>[8x]MTSVTSKQSTILGSDEIDLGRVIGELIDHRKLIISITSVFTLFAILYALLATPIYETDALIQIEQKQGNAILSSLSQVLPDGQPQSAPETALLQSRMILGKTIDDLNLQIQIEQKYFPVIGRGLARLMGEKPGNIDITRLYLPDSDDISNNTPSIILTVKDKENYSINSDGIQLNGVVGTLLNEKGISLLVNEIDAKPGDQFVITQLPRLKAISDLLKSFSVADLGKDTGMLTLTLTGDNPKRISHILDSISQNYLAQNIARQAAQDAKSLEFLNQQLPKVRAELDSAEDKLNAYRKQKDSVDLNMEAKSVLDQIVNVDNQLNELTFREAEVSQLYTKEHPTYKALMEKRQTLQEEKSKLNKRVSSMPSTQQEVLRLSRDVESGRAVYLQLLNRQQELNIAKSSAIGNVRIIDNAVTDPNPVRPKKTIIIVIGVVLGLIVSVVLVLFQVFLRRGIESPEQLEEIGINVYASIPISEWLTKNARQSGKVRKNQSDTLLAVGNPADLAVEAIRGLRTSLHFAMMEAKNNVLMISGASPSAGMTFISSNLAATIAITGKKVLFIDADLRKGYAHKMFGHKNDKGLSEFLSGQAAAEMIIDKVEGGGFDYIGRGQIPPNPAELLMHPRFEQLLNWASQNYDLIIIDTPPILAVTDAAIIGRYAGTCLLVARFEKNTVKEIDVSMKRFEQSGVVVKGCILNGVVKKASSYYRYGHNHYGYSYYDKKHHHHHH

Gram-negative species couple polymerization with translocation across the periplasm and outer membrane and the master regulator of the system is the tyrosine autokinase, Wzc. The tyrosine autokinase domain forms the cytoplasm region, while the periplasmic region contains small folded motifs and helical bundles. Autophosphorylation of the tyrosine-rich C-terminus of Wzc results in disassembly of the octamer into multiply phosphorylated monomers. We propose that the cycling between phosphorylated monomer and dephosphorylated octamer regulates glycan polymerization and translocation.

Previous work showed that mutation of K540 in the Walker box abrogated Wzc phosphorylation. In contrast to phosphorylated and enzymatically-dephosphorylated protein, purified non-phosphorylated WzcK540M was homogeneous, oligomeric (based on molecular mass in gel filtration) and yielded discrete octameric particles in negatively-stained EM images. Although the data were processed in C1, much of the structure displayed eightfold symmetry and the application of C8 symmetry improved the resolution to 2.30 Å. The WzcK540M octamer is ~165 Å high (cytosol to periplasm) and 146 Å wide and possesses a large central cavity with side portals that open to the membrane bilayer. The transmembrane region of each Wzc monomer comprises two helices (α2 K31 to L50 and α12 I428 to F447), which form an X-like arrangement with multiple side-chain interactions between them. The resulting arrangement of the eight transmembrane helical pairs is unusual; they are not closely packed, and this creates oval-shaped portals (20 Å wide by 45 Å high) located between the pairs of the helices. The conserved tyrosine-rich region (Tyr 708, 713, 715 and 717) reaches into the active site of the neighbouring subunit with Y717 positioned at the active site. Y715 sits in a pocket, where it makes a hydrogen bond with E675 from the neighbouring subunit site. Approximately two-thirds of the surface area buried by the formation of octamer occurs in the cytosolic region, with the remainder arising from contacts between motif 1 of the periplasmic domain. The interaction between the C-terminal tyrosine-rich tail and the kinase active site of each neighbouring subunit buries around 440 Å2 surface area (of total 1200 Å2 buried).> MSTSPGLAFANLTLLLDVPQLPAIWAVNAWRELNGLFT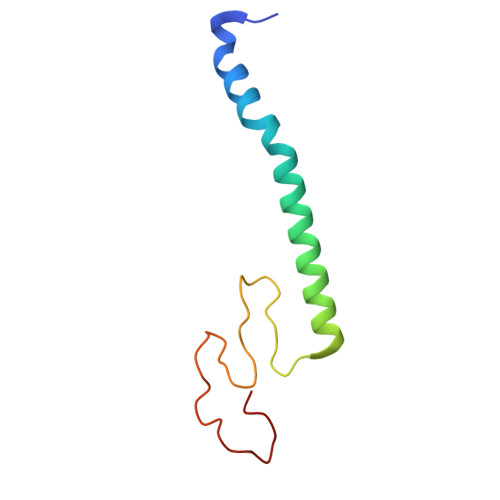EMKTLAGTSDLLYPSNRYNPQNEKTNRMGRPRKYNHGEWMFGNSY> AERPTLPIPDLLTTDARNRI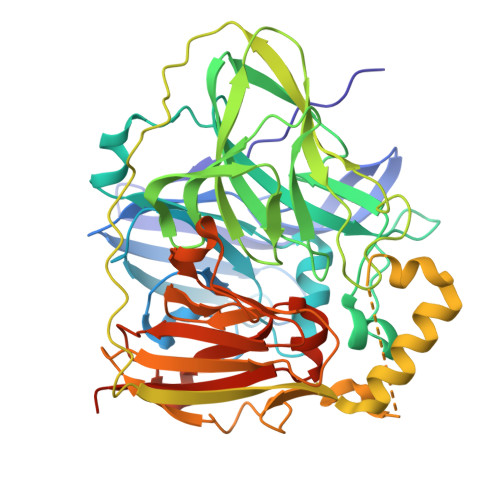QLTIGAGQSTFGGKTATTWGYNGNLLGPAVKLQRGKAVTVDIYNQLTEETTLHWHGLEVPGEVDGGPQGIIPPGGKRSVTLNVDQPAATCWFHPHQHGKTGRQVAMGLAGLVVIEDDEILKLMLPKQWGIDDVPVIVQDKKFSADGQIDYQLDVMTAAVGWFGDTLLTNGAIYPQHAAPRGWLRLRLLNGCNARSLNFATSDNRPLYVIASDGGLLPEPVKVSELPVLMGERFEVLVEVNDNKPFDLVTLPVSQMGMAIAPFDKPHPVMRIQPIAISASGALPDTLSSLPALPSLEGLTVRKLQLSMDPILDMMGMQMLMEKYGDQAMAGMDHSQMTSFAEYWALLSMNHGGKFDFHHANKINGQAFDMNKPMFAAAKGQYERWVISGVGDMMLHPFHIHGTQFRILSENGKPPAAHRAGWKDTVKVEGNVSEVLVKFNHDAPKEHAYMAHCHLLEHEDTGMMLGFTVKDPNSSSVDKLAAALEHHHHH>[2x]GMSARDV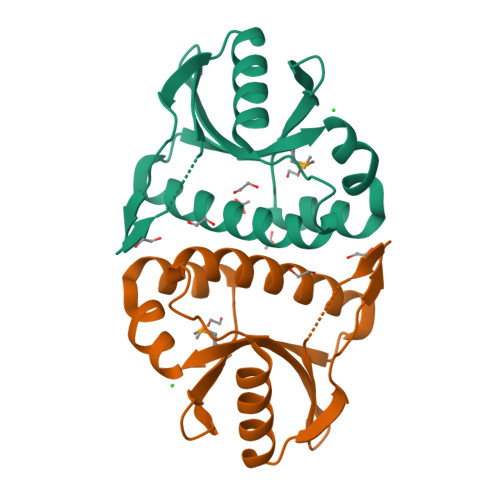FHEVVKTALKKDGWQITDDPLTISVGGVNLSIDLAAQKLIAAERQGQKIAVEVKSFLKQSSAISEFHTALGQFINYRGALRKVEPDRVLYLAVPLTTYKTFFQLDFPKEIIIENQVKMLVYDVEQEVIFQWIN>MAKEFGIPAAVAKTVLNVVEAGGWVTTIVSILTAVGSGGKSLLAAAGRESIKAYLKKEIKKKGKRAVIA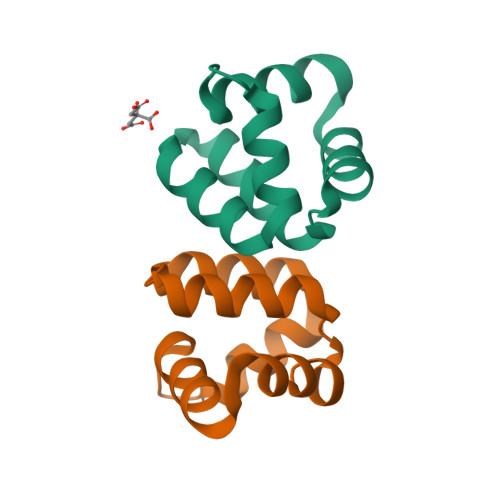W[2x]> IPEPKPGDLIEIFRPFYRHWAIYVGDGYVVHLAPPSEVAGAGAASVMSALTDKAIVKKELLYDVAGSDK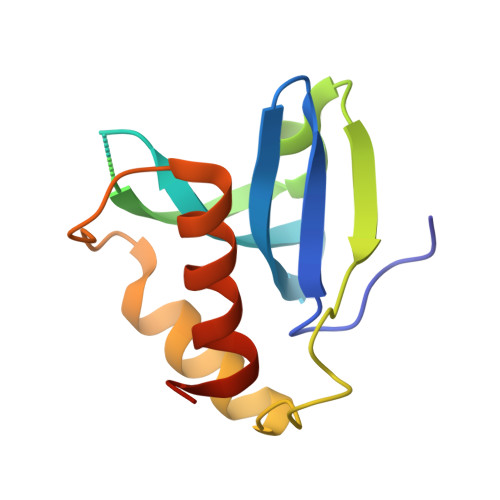YQVNNKHDDKYSPLPCSKIIQRAEELVGQEVLYKLTSENCEHFVNELRYGVAHHHHHH>MSSTPSNQNIIPIIKKESIVSLFEKGIRQDGRKLTDYRPLSITLDYAKKADGSALVKLGTTMVLAGTKLEIDKPYEDTPNQGNLIVNVELLPLAYETFEPGPPDENAIELARVVDRSLRDSKALDLTKLVIEPGKSVWTVWLDVYVLDYGGNVLDACTLASVAALYNTKVYKVEQHSNGISVNKNEVVGKLPLNYPVVTISVAKVDKYLVVDPDLDEESIMDAKISFSYTPDLKIVGIQKSGKGSMSLQDIDQAENTARSTAVKLLEELKKHLGI[12x];>[12x]MREMLQVERPKLILDDGKRTDGRKPDELRSIKIELGVLKNADGSAIFEMGNTKAIAAVYGPKEMHPRHLSLPDRAVLRVRYHMTPFSTDERKNPAPSRREIELSKVIREALESAVLVELFPRTAIDVFTEILQADAGSRLVSLMAASLALADAGIPMRDLIAGVAVGKADGVIILDLNETEDMWGEADMPIAMMP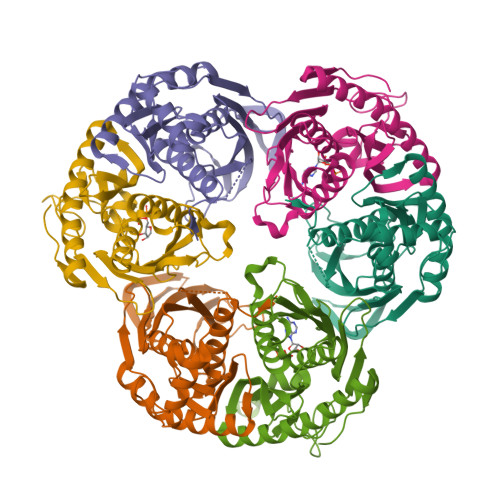SLNQVTLFQLNGSMTPDEFRQAFDLAVKGINIIYNLEREALKSKYVEFKEEGV>MKQFEIVIEPIQTEQYREFTINEYQGAVVVFTGHVREWTKGVKTEYLEYEAYIPMAEKKLAQIGDEINEKWPGTITSIVHRIGPLQISDIAVLIAVSSPHRKDAYRANEYAIERIKEIVPIWKKEIWEDGSKWQGHQKGNYEEAKREE[4x];>[4x]MKVLYFAEIKDILQKAQE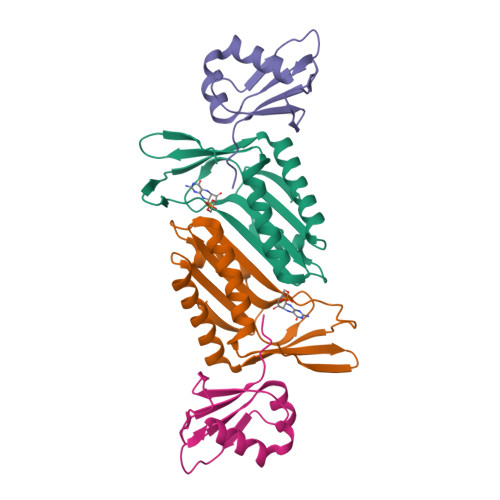DIVLEQALTVQQFEDLLFERYPQINNKKFQVAVNEEFVQKSDFIQPNDTVALIPPVSGG1-[[1-[(4-bromophenyl)methyl]-1,2,3-triazol-4-yl]methylamino]-2-methyl-1-oxidanylidene-propane-2-sulfonic acid | C14 H17 Br N4 O4 S | 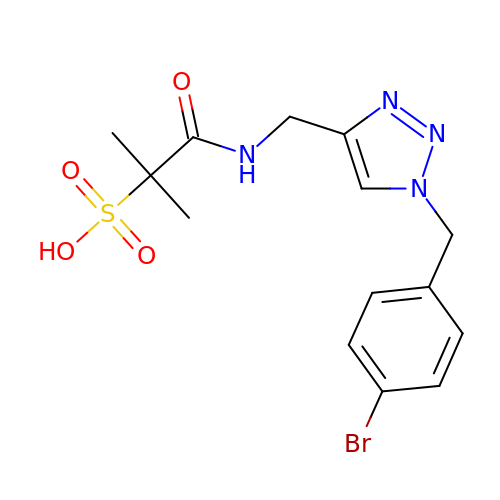MXYSCNLKJAGAQI-UHFFFAOYSA-N>[2x]GSHMASTTPLPLEPIETASRDELTALQLERLKWSLRHAYDHSPVYRRKFDEAGVHPDDLKTLADLSRFPFTTKGDLRDSYPFGMFAVPQDRI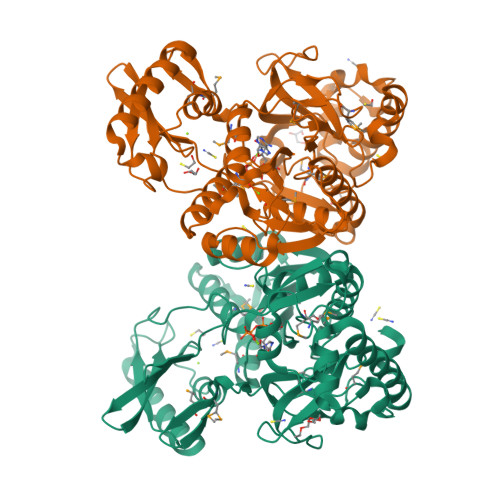SRIHASSGTTGKPTVVGYTAADIDTWANLVARSIRAAGARRGDKVHVSYGYGLFTGGLGAHYGAERAGLTVIPFGGGQTEKQVQLIQDFRPDIIMVTPSYMLSIADEIERQGLDPVQSSLRIGIFGAEPWTNDMRVAIEQRMGIDAVDIYGLSEVMGPGVASECVETKDGPTIWEDHFYPEIIDPETGEVLPDGELGELVFTSLTKEALPIIRYRTRDLTRLLPGTARTMRRMEKITGRSDDMMIVRGVNVFPTQIEEQLLKQRALAPHYQIVLTKEGPLDVLTLNVEPCPETAPDTAAIQVAKQALAYDIKSLIGVTAVINVLPVNGIERSVGKARRVVDKRKG> MENGYTYEDYKNTAEWLLSHTKHRPQVAIICGSGLGGLTDKLTQAQIFDYSEIPNFPRSTVPGHAGRLVFGFLNGRACVMMQG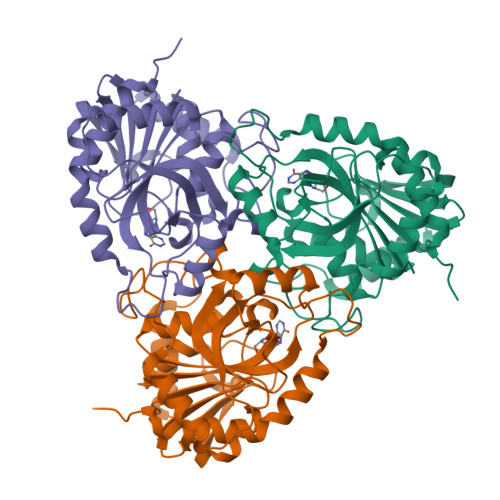RFHMYEGYPLWKVTFPVRVFHLLGVDTLVVTNAAGGLNPKFEVGDIMLIRDHINLPGFSGQNPLRGPNDERFGDRFPAMSDAYDRTMRQRALSTWKQMGEQRELQEGTYVMVAGPSFETVAECRVLQKLGADAVGMSTVPEVIVARHCGLRVFGFSLITNKVIMDYESLEKANFEEVLAAGKQAAQKLEQFVSILMASIPLPDKAS>MEPHVLGAVLYWLLLPCALLAACLLRFSGLSLVYLLFLLLLPWFPGPTRCGLQGHTGRLLRALLGLSLLFLVAHLALQICLHIVPRLDQLLGPSCSRWETLSRHIGVTRLDLKDIPNAIRLVAPDLGILVVSSVCLGICGRLARNTRQSPHPRELDDDERDVDASPTAGLQEAATLAPTRRSRLAARFRVTAHWLLVAAGRVLAVTLLALAGIAHPSALSSVYLLLFLALCTWWACHFPISTRGFSRLCVAVGCFGAGHLICLYCYQMPLAQALLPPAGIWARVLGLKDFVGPTNCSSPHALVLNTGLDWPVYASPGVLLLLCYATASLRKLRAYRPSGQRKEAAKGYEARELELAELDQWPQERESDQHVVPTAPDTEADNCIVHELTGQSSVLRRPVRPKRAEPREASPLHSLGHLIMDQSYVCALIAMMVWSITYHSWLTFVLLLWACLIWTVRSRHQLAMLCSPCILLYGMTLCCLRYVWAMDLRPELPTTLGPVSLRQLGLEHTRYPCLDLGAMLLYTLTFWLLLRQFVKEKLLKWAESPAALTEVTVADTEPTRTQTLLQSLGELVKGVYAKYWIYVCAGMFIVVSFAGRLVVYKIVYMFLFLLCLTLFQVYYSLWRKLLKAFWWLVVAYTMLVLIAVYTFQFQDFPAYWRNLTGFTDEQLGDLGLEQFSVSELFSSILVPGFFLLACILQLHYFHRPFMQLTDMEHVSLPGTRLPRWAHRQDAVSGTPLLREEQQEHQQQQQEEEEEEEDSRDEGLGVATPHQATQVPEGAAKWGLVAERLLELAAGFSDVLSRVQVFLRRLLELHVFKLVALYTVWVALKEVSVMNLLLVVLWAFALPYPRFRPMASCLSTVWTCVIIVCKMLYQLKVVNPQEYSSNCTEPFPNSTNLLPTEISQSLLYRGPVDPANWFGVRKGFPNLGYIQNHLQVLLLLVFEAIVYRRQEHYRRQHQLAPLPAQAVFASGTRQQLDQDLLGCLKYFINFFFYKFGLEICFLMAVNVIGQRMNFLVTLHGCWLVAILTRRHRQAIARLWPNYCLFLALFLLYQYLLCLGMPPALCIDYPWRWSRAVPMNSALIKWLYLPDFFRAPNSTNLISDFLLLLCASQQWQVFSAERTEEWQRMAGVNTDRLEPLRGEPNPVPNFIHCRSYLDMLKVAVFRYLFWLVLVVVFVTGATRISIFGLGYLLACFYLLLFGTALLQRDTRARLVLWDCLILYNVTVIISKNMLSLLACVFVEQMQTGFCWVIQLFSLVCTVKGYYDPKEMMDRDQDCLLPVEEAGIIWDSVCFFFLLLQRRVFLSHYYLHVRADLQATALLASRGFALYNAANLKSIDFHRRIEEKSLAQLKRQMERIRAKQEKHRQGRVDRSRPQDTLGPKDPGLEPGPDSPGGSSPPRRQWWRPWLDHATVIHSGDYFLFESDSEEEEEAVPEDPRPSAQSAFQLAYQAWVTNAQAVLRRRQQEQEQARQEQAGQLPTGGGPSQEVEPAEGPEEAAAGRSHVVQRVLSTAQFLWMLGQALVDELTRWLQEFTRHHGTMSDVLRAERYLLTQELLQGGEVHRGVLDQLYTSQAEATLPGPTEAPNAPSTVSSGLGAEEPLSSMTDDMGSPLSTGYHTRSGSEEAVTDPGEREAGASLYQGLMRTASELLLDRRLRIPELEEAELFAEGQGRALRLLRAVYQCVAAHSELLCYFIIILNHMVTASAGSLVLPVLVFLWAMLSIPRPSKRFWMTAIVFTEIAVVVKYLFQFGFFPWNSHVVLRRYENKPYFPPRILGLEKTDGYIKYDLVQLMALFFHRSQLLCYGLWDHEEDSPSKEHDKSGEEEQGAEEGPGVPAATTEDHIQVEARVGPTDGTPEPQVELRPRDTRRISLRFRRRKKEGPARKGAAAIEAEDREEEEGEEEKEAPTGREKRPSRSGGRVRAAGRRLQGFCLSLAQGTYRPLRRFFHDILHTKYRAATDVYALMFLADVVDFIIIIFGFWAFGKHSAATDITSSLSDDQVPEAFLVMLLIQFSTMVVDRALYLRKTVLGKLAFQVALVLAIHLWMFFILPAVTERMFNQNVVAQLWYFVKCIYFALSAYQIRCGYPTRILGNFLTKKYNHLNLFLFQGFRLVPFLVELRAVMDWVWTDTTLSLSSWMCVEDIYANIFIIKCSRETEKKYPQPKGQKKKKIVKYGMGGLIILFLIAIIWFPLLFMSLVRSVVGVVNQPIDVTVTLKLGGYEPLFTMSAQQPSIIPFTAQAYEELSRQFDPQPLAMQFISQYSPEDIVTAQIEGSSGALWRISPPSRAQMKRELYNGTADITLRFTWNFQRDLAKGGTVEYANEKHMLALAPNSTARRQLASLLEGTSDQSVVIPNLFPKYIRAPNGPEANPVKQLQPNEEADYLGVRIQLRREQGAGATGFLEWWVIELQECRTDCNLLPMVIFSDKVSPPSLGFLAGYGIMGLYVSIVLVIGKFVHGFFSEISHSIMFEELPCVDRILKLCQDIFLVRETRELELEEELYAKLIFLYRSPETMIKWTREKE[3x];>MSGAGEALAPGPVGPQRVAEAGGGQLGSTAQGKCDKDNTEKDITQATNSHFTHGEMQDQSIWGNPSDGELIRTQPQRLPQLQTSAQVPSGEEIGKIKNGHTGLSNGNGIHHGAKHGSADNRKLSAPVSQKMHRKIQSSLSVNSDISKKSKVNAVFSQKTGSSPEDCCVHCILACLFCEFLTLCNIVLGQASCGICTSEACCCCCGDEMGDDCNCPCDMDCGIMDACCESSDCLEICMECCGICFPS[3x]

PIEZO channels transmit mechanical force signals to cells, allowing them to make critical decisions during development and in pathophysiological conditions. Here, we report several near-atomic resolution cryo-EM structures of fast-inactivating wild-type human PIEZO1 (hPIEZO1) and its slow-inactivating channelopathy mutants with or without its auxiliary subunit MDFIC. Each hPIEZO1 subunit has a curved blade structure, and the three subunits form the trimeric PIEZO channel, exhibiting a bowl-like shape. MDFIC, a MyoD family inhibitor protein, has recently been identified as an auxiliary subunit of piezo channels capable of decelerating channel inactivation and attenuating channel mechanosensitivity.

While the severe hereditary erythrocytosis mutant R2456H significantly slows down the inactivation of hPIEZO1, the hPIEZO1-R2456H-MDFIC complex shows a more curved and contracted structure with an inner helix twist due to the broken link between the pore lipid and R2456H. For hPIEZO1-R2456H-MDFIC, the 2D class averages show a clear trimer state. The resolution of hPIEZO1-R2456H-MDFIC was improved to 4.6 Å with 16K particles, allowing us to build a relatively accurate model of the transmembrane helices based on the hPIEZO1-MDFIC model (Figure 5—figure supplements 2 and 3). On the other hand, the hPIEZO1-R2456H-MDFIC shows a smaller disk of 25 nm compared to the 30 nm for the wild type and the other two mutants. The smaller disk is mainly due to the more significant contraction of the blade arms and a more curved state compared to the wild-type hPIEZO1-MDFIC in the side view. Surprisingly, the IH of hPIEZO1-R2456H-MDFIC showed a significant twist of ~35° compared to wild-type hPIEZO1-MDFIC. The coiled-coil shape of the IH pore results in a more dilated pore on the extracellular side, suggesting that unlike the mild GOF E756del and A1988V mutations present in the typical African population and located in the THUs region, the more severe mutation R2456H, which is located in the IH, not only leads to blade reshaping but also results in pore expansion. The hPIEZO1-R2456H-MDFIC presents a more extended extracellular side pore. More robust evidence comes from the HX channelopathy mutant R2456H, wherein the interaction between the hydrophilic phosphate group head and R2456 is disrupted, which leads to remodeling of the blade and pore module, thus significantly prolonging the inactivation time. Due to the stabilizing effect of the MDFIC auxiliary subunit, the pore has a twisted shape, and the overall architecture of hPIEZO1-R2456H-MDFIC has a more curved and contracted bowl-like shape.(5R)-3-tert-butyl-1-(6-chloro-1,3-benzothiazol-2-yl)-4,5-dihydro-1H-pyrazol-5-ol 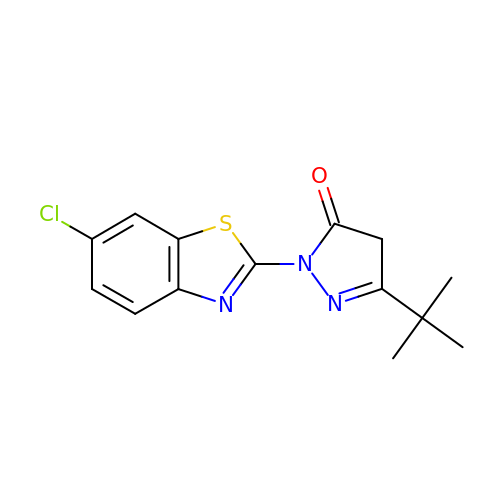| C14 H14 Cl N3 O S | PZAXHXFHBHHFNG-UHFFFAOYSA-N>KEENNFINLYTVKNPLKCKIVDKINLVRPNSP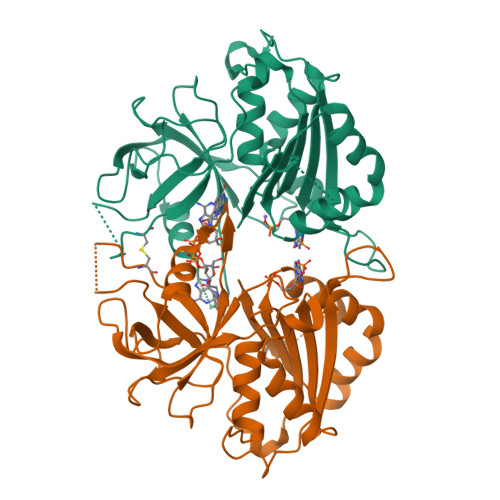NEVYHLEINHNGLFKYLEGHTCGIIPYYNELDNNPNNQINKDHNIINTTNHTNHNNIALSHIKKQRCARLYSISSSNNMENLSVAIKIHKYEQTENAPNITNYGYCSGFIKNLKINDDIYLTGAHGYFNLPNDAIQKNTNFIFIATGTGISPYISFLKKLFAYDKNNLYNRNSNYTGYITIYYGVYNEDSILYLNELEYFQKMYPNNINIHYVFSYKQNSDATSFYVQDEIYKRKTEFLNLFNNYKCELYICGHKSIRYKVMDILKSHDQFDEKKKKRVHVEVY[6x]>[2x]MHHHHHHMAHFMDVHRGMHGITSDQLHQAH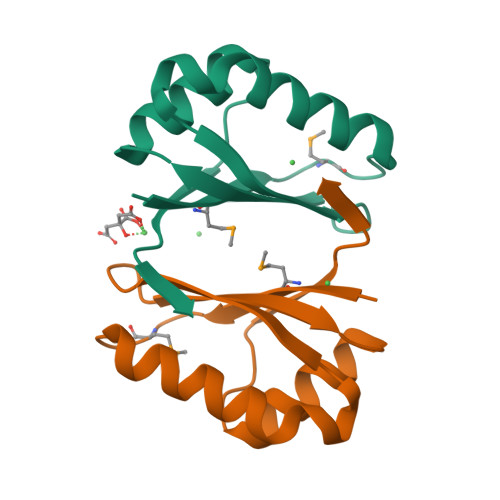QADLAVEKDENVHFEQAWADPASGTIYCLSEGPSAEAVQRVHERAGHKADEIHEVPLSA(S)-2-CHLORO-N-(1-(2-(2-HYDROXYETHYLAMINO)-2-OXOETHYL)-2-OXO-1,2,3,4-TETRAHYDROQUINOLIN-3-YL)-6H-THIENO[2,3-B]PYRROLE-5-CARBOXAMIDE | C20 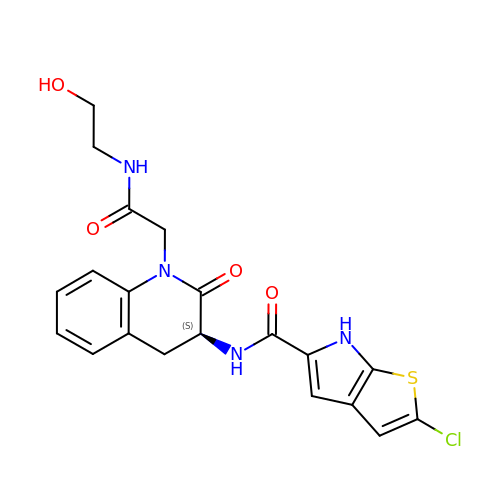H19 Cl N4 O4 S | VUKPNWLGSLOHIF-AWEZNQCLSA-N>ATWTCINQQLNPKTNKWEDKRLLYSQAKAESNSHHAPLSDGKTGSSYPHWFTNGYDGNGKLIKGRTPIKFGKADCDRPPKHSQNGMGKDDHYLLEFPTFPDGHDYKFDSKKPKEDPGPARVIYTY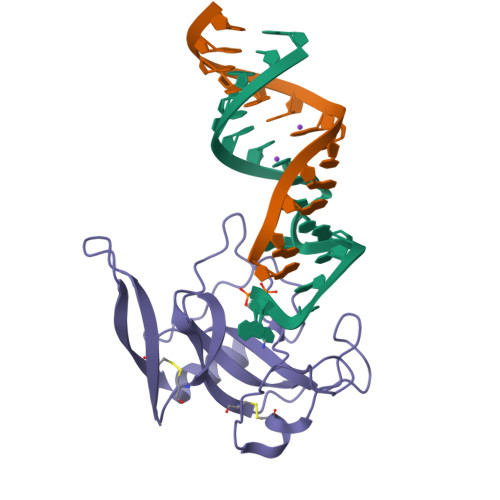PNKVFCGIVAHQRGNQGDLRLCSH[2x]> MDIVKLRELLEAELSSTDLNELDEDFYVEFDSLIKALKLSAESSRERGEDVEERLYLAQLKIAESLMK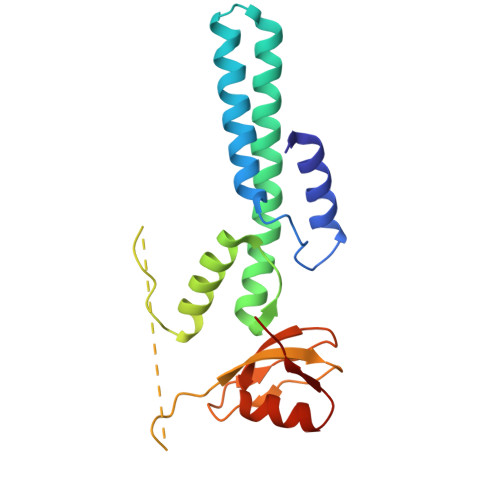EIIKLRLHKIVDLAVEGKIAEMTAEEKRLFNVIRAFIEREELPEISEEVQPQEESEAEAEYRSKEVPKEAYIIQIDLPAVLGPDMKEYGPFMAGDMAIIPTVIGRALVEREAARRVRIFL> MANKTEKPTPKKLKDAAKKGQSFK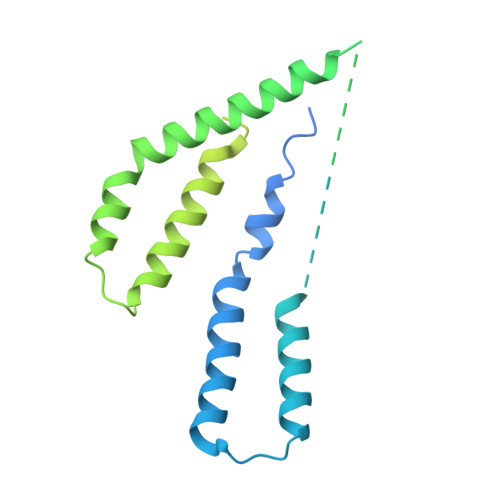FKDLTTVVIILVGTFTIISFFSLSDVMLLYRYVIINDFEINEGKYFFAVVIVFFKIIGFPLFFCVLSAVLPTLVQTKFVLATKAIKIDFSVLNPVKGLKKIFSIKTIKEFFKSILLLIILALTTYFFWINDRKIIFSQVFSSVDGLYLIWGRLFKDIILFFLAFSILVIILDFVIEFILYMKDMMMDKQEIKREYIEQEGHFETKSRRRELHIEILSEQTKSDIRNSKLVVMNPTHIAIGIYFNPEIAPAPFISLIETNQCALAVRKYANEVGIPTVRDVKLARKLYKTHTKYSFVDFEHLDEVLRLIVWLEQVENTH>[2x]SETQSFVVSVAGSDRVGIVHDFSWA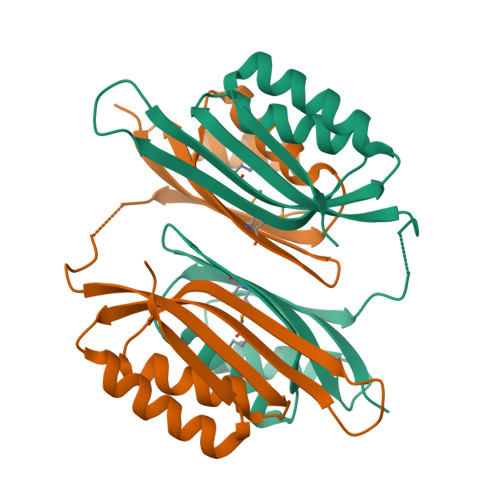LKNISANVESSRMACLGGDFAMIVLVSLNAKDGKLIQSALESALPGFQISTRRASSVAERHVSPDTREYELYVEGPDSEGIVEAVTAVLAKKGANIVELETETLPAPFAGFTLFRMGSRVAFPFPLYQEVVTALSRVEEEFGVDIDLEEVVEGEDSEEDDDSPNSPVGRH>VSSRVSTRSSLAEDLRAIGLADGDAVLVAAALRKVGKIVGGPDDILDAMRDVIGPAGTVLGYADWQLEDEIRDDPAMREHIPAFDPLRSRSIRDNGFWPELIRTTPGALRSASPGASMAAIGGEAEWFTADHALDYGYGPRSPLGKLVEAKGKVLMLGAPLDTMTLLHHA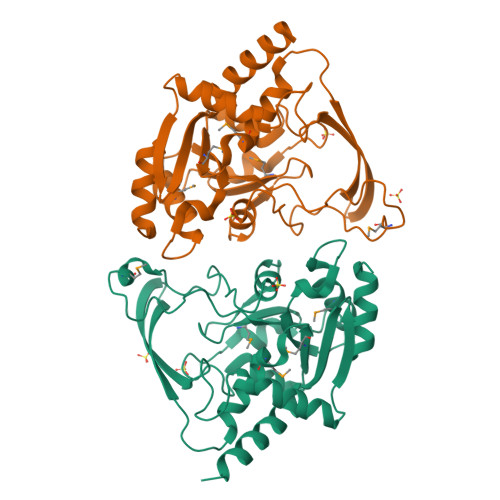EHLADFPNKRILRYEAPILVDGEKVWRWFEEFDTSDPPDGLADDYFAGIVEEFLATGRGKRGKIGEASSVLVPADEIVAFAVDWLERWGRTAR[6x]>MSNIQNMSLEDIMGERFGRYSKYIIQDRALPDIRDGLKPVQRRILYSMNKDSNTFDKSYRKSAKSVGNIMGNFHPHGDSSIYDAMVRMSQNWKNREILVEMHGNNGSMDGDPPAAMRYTEARLSEIAGYLLQDIEKKTVPFAWNFDDTEKEPTVLPAAFPNLLVNGSTGISAGYATDIPPHNLAEVIDAAVYMIDHPTAKIDKLMEFLPGPDFPTGAIIQGRDEIKKAYETGKGRVVVRSKTEIEKLKGGKEQIVITEIPYEINKANLVKKIDDVRVNNKVAGIAEVRDESDRDGLRIAIELKKDANTELVLNYLFKYTDLQINYNFNMVAIDNFTPRQVGIVPILSSYIAHRREVILARSRFDKEKAEKRLHIVEGLIRVISILDEVIALIRASENKADAKENLKVSYDFTEEQAEAIVTLQLYRLTNTDVVVLQEEEAELREKIAMLAAIIGDERTMYNLMKKELREVKKKFATPRLSSLEDTAKALEHHHHHH[2x];>[2x]MGHHHHHHHHHHSSGHIDDDDKHMKNKKDKGL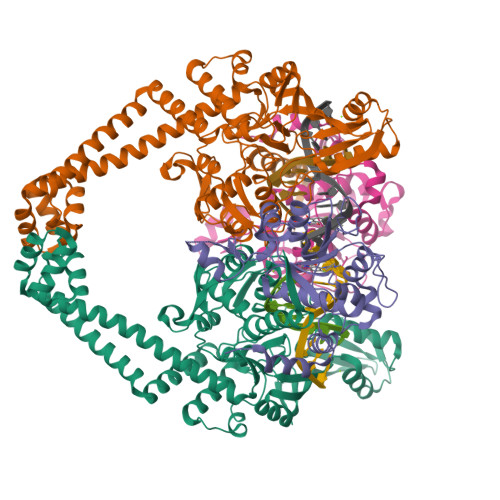LSGKLTPAQSKNPAKNELYLVEGDSAGGSAKQGRDRKFQAILPLRGKVINTAKAKMADILKNEEINTMIYTIGAGVGADFSIEDANYDKIIIMTDADTDGAHIQTLLLTFFYRYMRPLVEAGHVYIALPPLYKMSKGKGKKEEVAYAWTDGELEELRKQFGKGATLQRYKGLGEMNADQLWETTMNPETRTLIRVTIEDLARAERRVNVLMGDKVEPRRKWIEDNVKFTLEEATVF> RNLLTNGEGLYAGQSLDVEPYHFIMQEDCNLVLYDHSTSVWASNTGILGKKGCKAVLQSDGNFVVYDAEGRSLWASHSV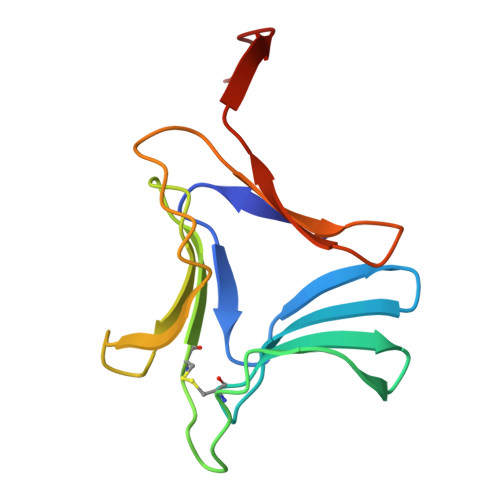RGNGNYVLVLQEDGNVVIYGSDIWSTGTYK N-benzyl-4-(pyridin-3-yl)pyrimidin-2-amine | 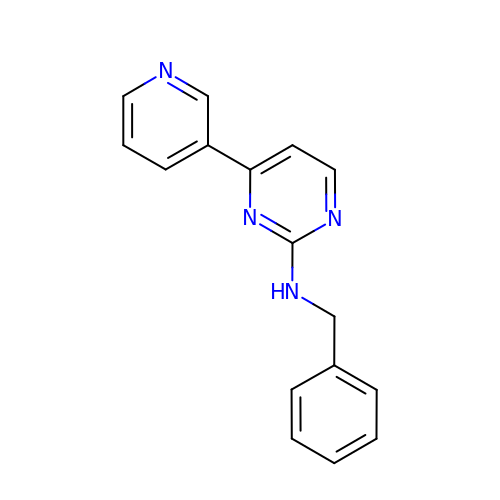C16 H14 N4 | JTYLHRZXSYVYMO-UHFFFAOYSA-N>GSHMASMSEVERALDVLLQEAEELCIGSSVVELDRIPTALEFCREFYSKNQPVVIRKALNWPAIGKWTPKYLIEALGDRSV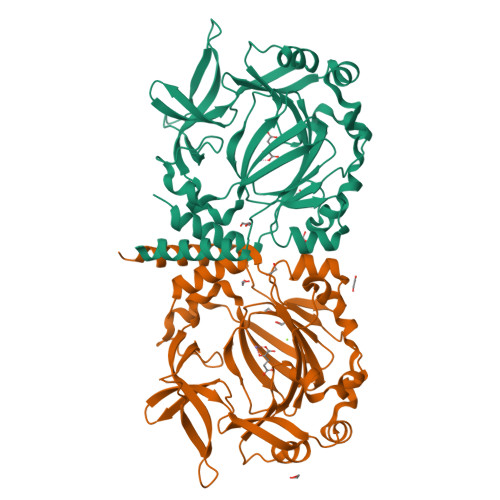DVAITPNGYADGLATQNGQEYFVLPLETKMKLSEVVRRLDDPTGAVHYIQKQNSNLSVDLPELAADLRVSDLDFAQQSFNKPPDAVNFWLGDERAVTSMHKDPYENVYCVISGHKDFVLIPPHQLSCVPRGIYPTGVYKTSDSGQFYIEPLRDEEGSDQFTEWVSVDPLSPDLAKYPEYARAKPLKVRVHAGDILYLPNYWFHHVSQSHKCIAVNFWYDLDYDSRYCYYRMLEQMTSARSG[2x]> GPMRTKIVVKVHMPCGKSR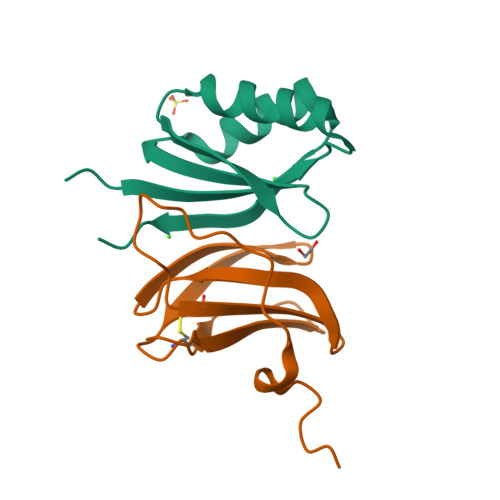AKAMALAASVNGVDSVEITGDDKDRLQVVGRGIDPVRLVALLREKCGLAELLQVEEVKE;> GPMRAIDLSRERDPNFFDNADIPVPECFWFMFKNNVRQDAGTCYSSWKMDKKVGPNWVHIKSDDNCNLSGDFPPGWIVLGKKRPGF4-[[3-[2-chloranyl-6-(trifluoromethyl)phenyl]-5-(1~{H}-pyrrol-3-yl)-1,2-oxazol-4-yl]methoxy]-2-fluoranyl-benzoic acid | C22 H13 Cl F4 N2 O4 | 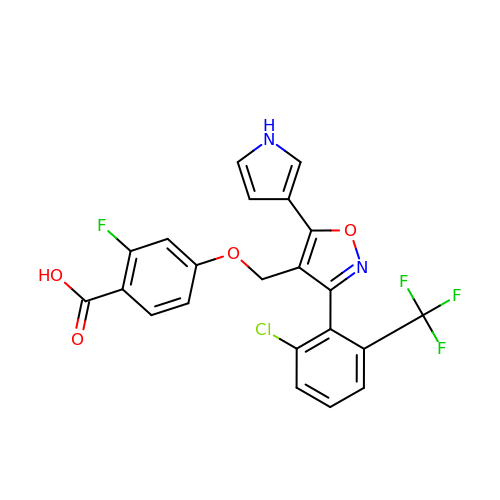WKGLEAWUJDYKCF-UHFFFAOYSA-N> MYPPKFGYVIPDNLNEALEFLEEHQDARPLAGGHSLIPMLKLRLIRPSYIVEIRRFSNLSYITKDGNLYKIGALTTHYNISKSSIPLLSETASNIGDPQVRNMGTIGGSISHLDPSADYPAALIAMDAKVKITSRKGDRVVNFKSFAKDMFTPDLNPGELVTEIQVPTFEGYKFSYQKLERRAGDFAIVGVALLLKLSGDVIEDVRIGLTAVNNVAVRAKGAEEELLGKRLNDEIIEKAATR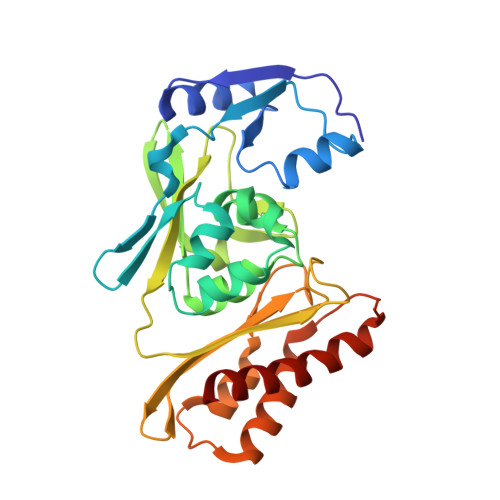AMESANPTSDLRGSAEYKKKMVKVLTKRAIITALKR> GSMDPAIYFKEQFLDGDAWTNRWVESKHKSDFGKFVLSSGKFYGDLEKDKGLQTSQDARFYALSAKFEPFSNKGQTLVVQFTVKHEQNIDCGGGYVKLFPSGLDQKDMHGDSEYNIMFGPDICGPGTKKVHVIFNYKG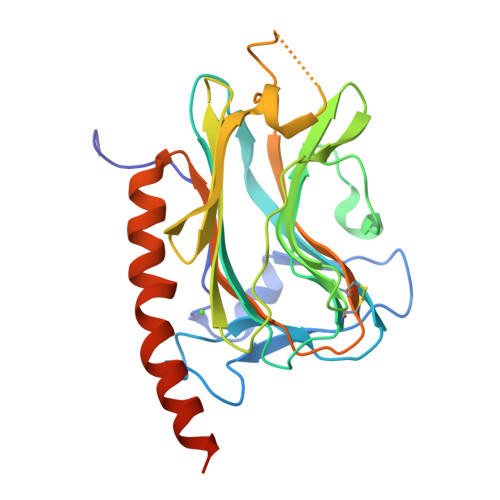KNVLINKDIRSKDDEFTHLYTLIVRPDNTYEVKIDNSQVESGSLEDDWDFLPPKGSGSGPDANIYAYDSFAVLGLDLWQVKSGTIFDNFLITNDEAYAEEFGNETWGVTKAAEKQMKDKQDEEQRLKLEHHHHHH> MLSFLWDLASFIVALGVLITVHEFGHFWVARRCGVRVERFSIGFGKALWRRTDKLGTEYVIALIPLGGYVKMLDERAEPVVPELRHHAFNNKSVGQRAAIIAAGPVANFIFAIFAYWLVFIIGVPGVRPVVGEIAANSIAAEAQIAPGTELKAVDGIETPDWDAVRLQLVDKIGDESTTITVAPFGSDQRRDVKLDLRHWAFEPDKEDPVSSLGIRPRGPQIEPVLENVQPNSAASKAGLQAGDRIVKVDGQPLTQWVTFVMLVRDNPGKSLALEIERQGSPLSLTLIPESKPGNGKAIGFVGIEPKVIPLPDEYKVVRQYGPFNAIVEATDKTWQLMKLTVSMLGKLITGDVKLNNLSGPISIAKG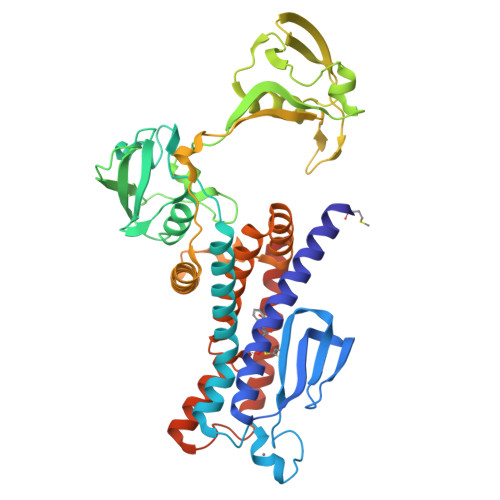AGMTAELGVVYYLPFLALISVNLGIINLFPLPVLDGGHLLFLAIEKIKGGPVSERVQDFCYRIGSILLVLLMGLALFNDFSRLGTENLYFQ>RLYWDDLKRKLSEKLDSTDFTSTIKLLNENSYVPREAGSQKDENLALYVENQFREFKLSKVWRDQHFVKIQVKDSAQNSVIIVDKNGRLVYLVENPGGYVAYSKAATVTGKLVHANFGTKKDFEDLYTPVNGSIVIVRAGKITFAEKVANAESLNAIGVLIYMDQTKFPIVNAELSFFGHAHLGTGDPYTPGFPSFNHTQFPPSRSSGLPNIPVQTISRAAAEKLFGNMEGDCPSDWKTDSTCRMVTSESKNVKLTVSNVLKEIKILNIFGVIKGFVEPDHYVVVGAQRDAWGPGAAKSGVGTALLLKLAQMFSDMVLKDGFQPSRSIIFASWSAGDFGSVGATEWLEGYLSSLHLKAFTYINLDKAVLGTSNFKVSASPLLYTLIEKTMQNVKHPVTGQFLYQDSNWASKVEKLTLDNAAFPFLAYSGIPAVSFCFCEDTDYPYLGTTMDTYKELIERIPELNKVARAAAEVAGQFVIKLTHDVELNLDYERYNSQLLSFVRDLNQYRADIKEMGLSL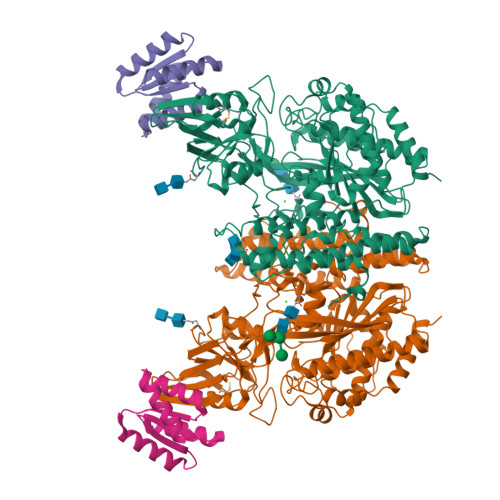QWLYSARGDFFRATSRLTTDFGNAEKTDRFVMKKLNDRVMRVEYHFLSPYVSPKESPFRHVFWGSGSHTLPALLENLKLRKQNNGAFNETLFRNQLALATWTIQGAANALSGDVWDIDNEF[2x];>DEEEIQKAIEELLRKGVSEEEAAIIIVQRFNVAVVVVVQDERQGKHISEYIRRYIPEADVILFANLVVIKVETHELSTRVWEAAQKAY[2x]>GSHMEQRILKFLEELGEGKATTAHDLSGKLGTPKKEINRVLY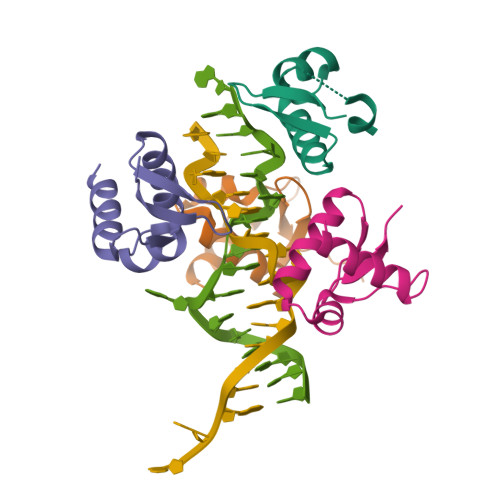SLAKKGKLQKEAGTPPLWKIAVSTQ[4x]> SANKVTKNKSNS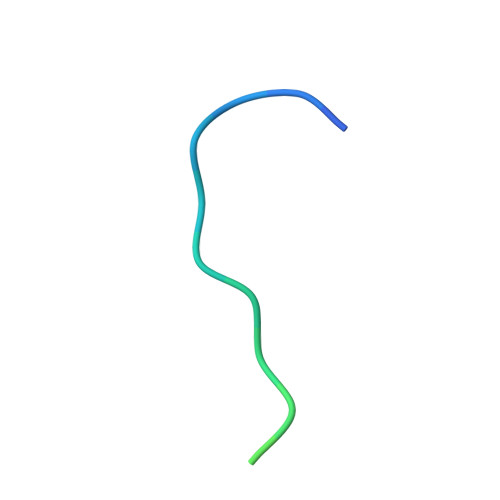SPYLNKRRGKPGPDS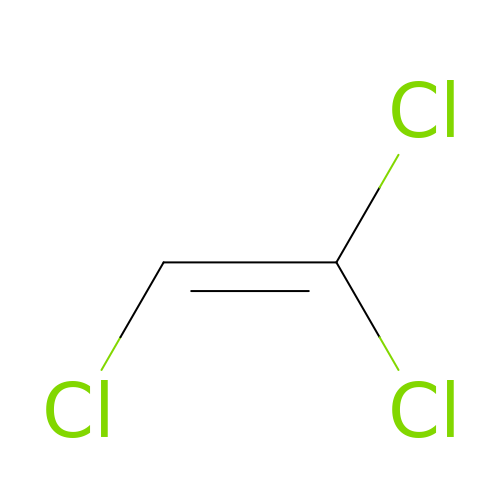1,1,2-trichloroethene | C2 H Cl3 | XSTXAVWGXDQKEL-UHFFFAOYSA-N> VTPPCTQERHYEHLGRCCSRCEPGKYLSSKCTPTSDSVCLPCGPDEYLDTWNEEDKCLLHKVCDAGKALVAVDPGNHTAPRRCACTAGYHWNSDCECCRRNTECAPGFGAQHPLQLNKDTVCTPCLLGFFSDVFSSTDKCKPWTNCTLLGKLEAHQGTTE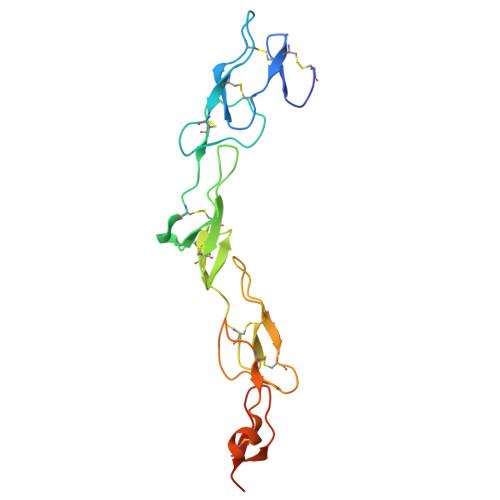SDVVCSSSGSLVPR>NLIPTVIEQTNRGERAYDIYSRLLKDRIIMLGSAIDDNVANSIVSQLLFLAAEDPEKEISLYINSPGGSITAGMAIYDTMQFIKPKVSTICIGMAASMGAFLLAAGEKGKRYALPNSE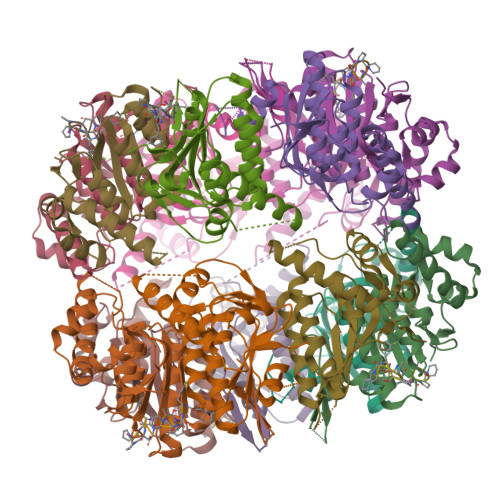VMIHQPLGGAQGQATEIEIAAKRILLLRDKLNKVLAERTGQPLEVIERDTDRDNFKSAEEALEYGLIDKILTHLEHHHHHH[28x]>[2x]MAGILEMVARGWKYFSGNFYYFSRTPKTWYSAEQFCISRKAHLTSVSSESEQKFLYKAADGIPHWIGLTKAGSEGDWYWVDQTSFNKEQSRRFWIPGEPNNAGNNEHCANIRVSALK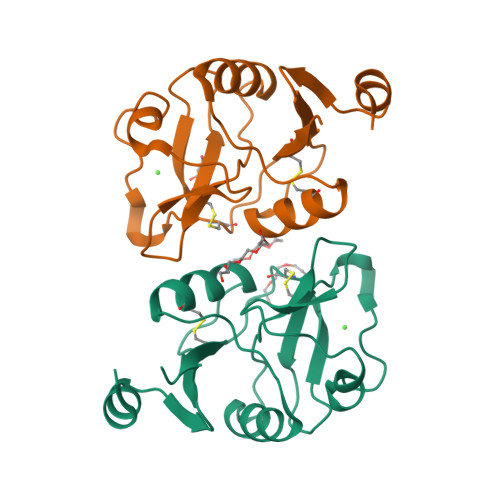CWNDGPCDNTFLFICKRPYVQTTEGTWSHPQFEK> MTADRPALRTGDRDTRLSFGSNLS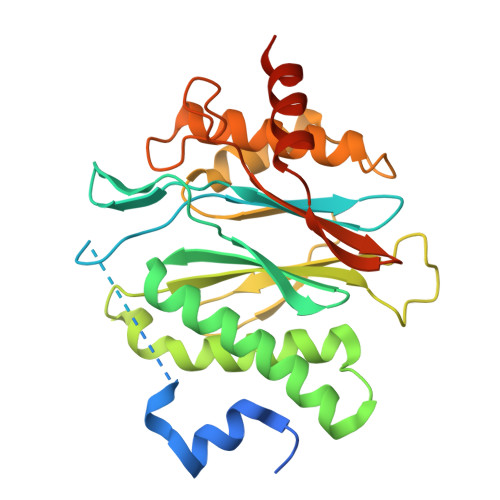SFTDYLRGHAPELLPENRIGHRSHSTRGGDGMESGDLAPHGTTIVALTYKGGVLLAGDRRATQGNLIASRDVEKVYVTDEYSAAGIAGTAGIAIELVRLFAVELEHYEKIEGVPLTFDGKANRLASMVRGNLGAAMQGLAVVPLLVGYDLDADDESRAGRIVSYDVVGGRYEERAGYHAVGSGSLAAKSALKKIYSPDSDEETALRAAIESLYDAADDDSATGGPDLTRGIYPTAVTITQAGAVHVSEETTSELARRIVAERTEQGGSAR> GSHMSPREQDRFLPIANVS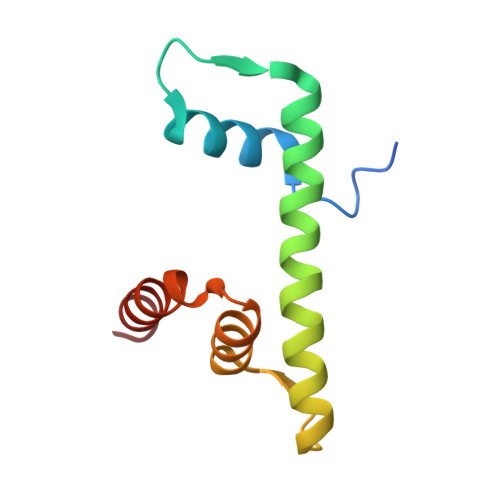RIMKKALPANAKISKDAKETMQECVSEFISFVTGEASDKCQKEKRKTINGDDLLWAMTTLGFEDYVEPLKVYLQRFRE>[2x]MHAALSPLSQRFERIAVQPLTGVLGAEITGVDLREPLDDSTWNEILDAFHTYQVIYFPGQAITNEQHIAFSRRFGPVDPVPLLKSIEGYPEVQMIRREANESGRVIGDDWHTDSTFLDAPPAAVVMRAIDVPEHGGDTGFLSMYTAWETLSPTMQATIEGLNVVHSATRVFGSLYQAQNRR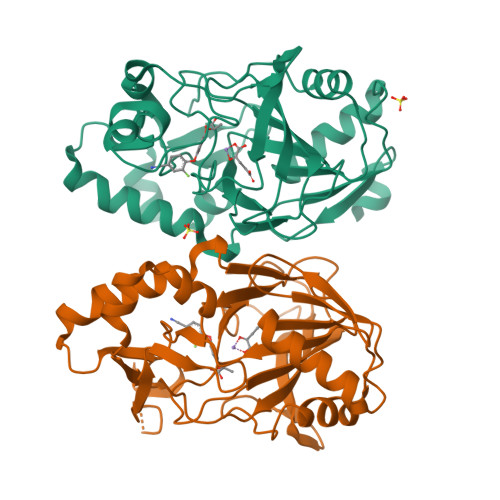FSNTSVKVMDVDAGDRETVHPLVVTHPGSGRKGLYVNQVYCQRIEGMTDAESKPLLQFLYEHATRFDFTCRVRWKKDQVLVWDNLCTMHRAVPDYAGKFRYLTRTTVGGVRPAR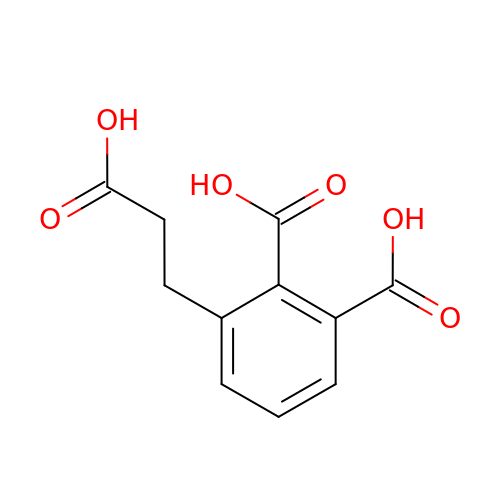3-(2-carboxyethyl)benzene-1,2-dicarboxylic acid | C11 H10 O6 | KVTUASDNLLIPPQ-UHFFFAOYSA-N> VIGDLKCTTVSINDVDTGAPSISTDTVDVTNGLGTYYVLDRVYLNTTLLLNGYYPTSGSTYRNMALKGTLLLSRLWFKPPFLSDFINGIFAKVKNTKVIKKGVMYSEFPAITIGSTFVNTSYSVVVQPHTTNLDNKLQGLLEISVCQYTMCEYPHTICHPKLGNKRVELWHWDTGVVSCLYKRNFTYDVNADYLYFHFYQEGGTFYAYFTDTGVVTKFLFNVYLGTVLSHYYVLP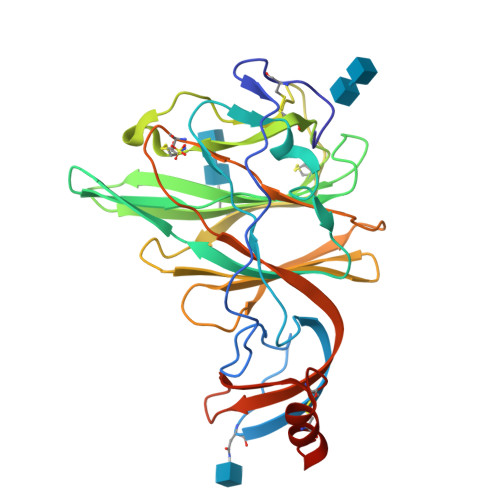LTCSSAMTLEYWVTPLTSKQYLLAFNQDGVIFNAVDCKSDFMSEIKCKTHHHHHH>[2x]S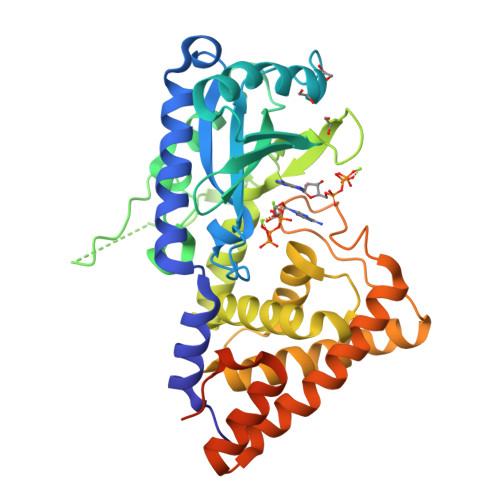MELQPQFNEFLANIRPTDTQKEDWKSGARTLRERLKNFEPLKEIVVSTFLQGSIRRSTAIRPLGDKRPDVDIVVVTNLDHTRMSPTDAMDLFIPFLEKYYPGKWETQGRSFGITLSYVELDLVITAIPESGAEKSHLEQLYKSESVLTVNSLEEQTDWRLNKSWTPNTGWLSESNSAQVEDAPASEWKAHPLVLPDREKNEWGRTHPLAQIRWTAEKNRLCNGHYINLVRAVKWWRQQNSEDLPKYPKGYPLEHLIGNALDNGTTSMAQGLVQLMDTFLSRWAAIYNQKSKPWLSDHGVAEHDVMARLTAEDFCSFYEGIASAAEIARNALASEEPQESAQLWRQLFGSKFPLPGPQGGDRNGGFTTPSKPAEPQKTGRFA> GAMGMTTDEGAKNNEESPTATVAEQGEDITSKKDRGVLKIVKRVGNGEETPMIGDKVYVHYKG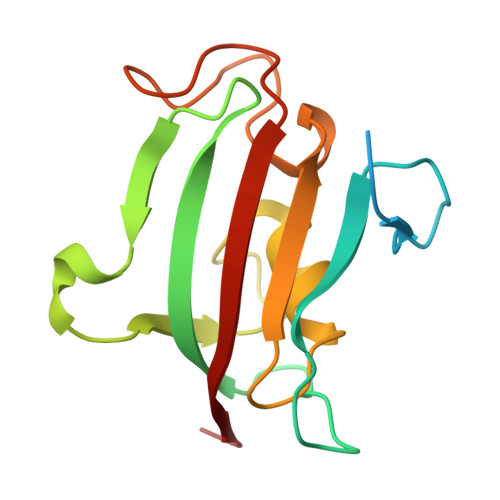KLSNGKKFDSSHDRNEPFVFSLGKGQVIKAWDIGVATMKKGEICHLLCKPEYAYGSAGSLPKIPSNATLFFEIELLDFKGE>[24x]SSQIRQNYSTDVEAAVNSLVNLYL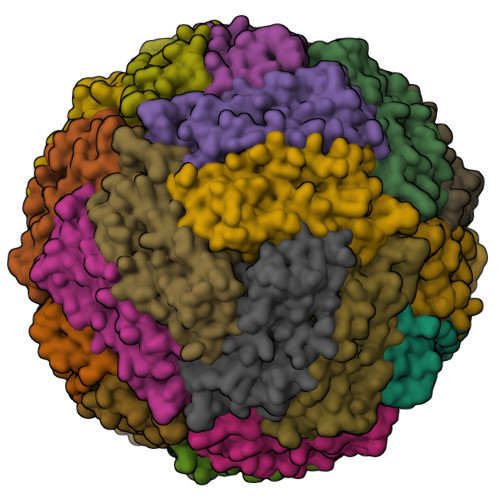QASYTYLSLGFYFDRDDVALEGVSHFFRELAEEKREGYERLLKMQNQRGGRALFQDIKKPAEDEWGKTPDAMKAAMALEKKLNQALLDLHALGSARTDPHLCDFLETHFLDEEVKLIKKMGDHLTNLHRLGGPEAGLGEYLFERLTLKHD>MYFFSVDPRNGASKSGDVCGSCCCESISARPGEVNGVMVSYAAWSAPLRGHGLTNKTTFEIDGVSVTPPKVSNAFGRTKVGVVFEGTLSDLFPNPEGEQVEYEISELNGPSNGVVELGANGAFTYTPGALFTGVDRFWFSINGNIGEYVISVDPTTSELPQPPFTTPVYVPAARRSVDPRTHVLKFVLGVSPAAIPGDVYRLTVRQVAIDCDGNEFVHISCYDISIGSCG[60x];>[12x]MLGIPLLTRKAALTPPAPSANPAKIFIRRFFSAGVAKNVVSYSNVMAAQRAMEHPVAFRCLDKLGLTVQSVKWDVGKDPQNTQVGDGGMSASQRKALQQILQRPNPTMSGAQLRYSAALSWACFGRMAFKVSVMSDGSVNAIWPLGIPFLKQKFDRYGDVESFQYGDEAGKETIPSFTKVEKNDKGRPIKNYAFMIVKPSINGAMNFDVQNTPLQAIGVPVALYDALMARAIDSADGTPNSKWLVTASRDLDDGQAKEVKEGIEETKPGGDNGGEIIFIAGTDVKVQEMKNDLSDIHSKVPLDDQARTIAGNFGIPIALLGFAGADGSKFANNYDESRKAFFEDTIEPGYLTPLEDGFSMFLCGAGYRVIFDRDSIPALRKSRADIAATYDKVTFITEEEKREVTGWPAKKEGQTQNDDA;>[6x]MRTADRKHRVIVCSQQSDVDDEGRLLITRAGVIQGWAAIAPVKAIRFSQDGVSMQKDTMQPTHDITMNYNPDVNVSVSAWVYEHRLKSPPRWFKVLSVVNVDECSRYMKIRCRLVETSDDVTPPVEEEKNSFGAVKIDIPL;>METKLTYGNRVTLPEFAKYIVAPAFHEIEGRAIPVTGVDDDASGTQATKLPFVLVGLRQGDTSGPATIAGNSTINLRDDFIVEFNMKKERYRDRKGGETPFFSYYDYESIRDRLFNSMIEFSGEHGITFEFVSLDISTEGDVVYIEFRFRQNYEWCETVREADTTIEAGRFSINLQGC[6x];>[6x]MACNKQNGVKNILITFTDCDTQEVIGPISHEQPDDTLPTYKNCAWTNTALTNGYVQRSASNATMTLPVVRDLRVPLAFYQGCAQVDVQVEKFDGTVMTLTEGAVVEPEE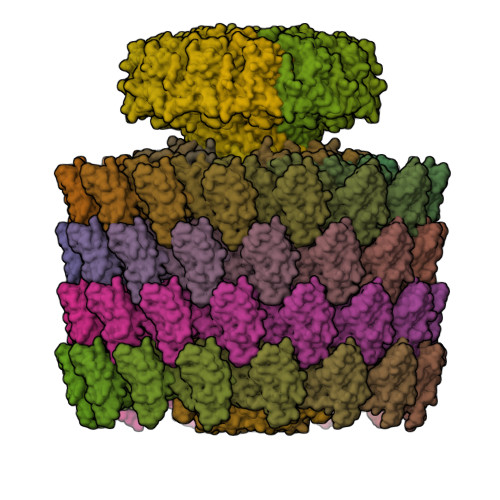SDGRSVTMNIVASEIDELLPPGSLAAA;>[12x]MNLDTLLPLQTIREHAKCDDNPRVTDDLLKLYREAAFEAAELYTGLSFTPEKTIVEPIRLKGRRGKIILSATPIAGRPVVFYGGGLGSPLELIPRPGSNVLFFPYGSPDRFQTWGDCHTCDVESQLMATYVTGRRCENSVPAGIIIGILKLIAWNINNPGDEVMSVRNTLNANAQGLIGGTNNGAVISGAQDEWFRYRRVLL>[4x]MLNSFKLSLQYILPKLWLTRLAGWGASKRAGWLTKLVIDLFVKYYKVDMKEAQKPDTASYRTFNEFFVRPLRDEVRPIDTDPNVLVMPADGVISQLGKIEEDKILQAKGHNYSLEALLAGNYLMADLFRNGTFVTTYLSPRDYHRVHMPCNGILREMIYVPGDLFSVNHLTAQNVPNLFARNERVICLFDTEFGPMAQILVGATIVGSIETVWAGTITPPREGIIKRWTWPAGENDGSVALLKGQEMGRFKLG;>XTVINLFAPGKVNLVEQLESLSVTKIGQPLAVSTGHHHHHHG[4x]

Phosphatidylethanolamine (PE), a major component of the cellular membrane across all domains of life, is synthesized exclusively by membrane-anchored phosphatidylserine decarboxylase (PSD) in most bacteria. PSD is translated as an inactive proenzyme and undergoes self-cleavage between a conserved Gly-Ser pair to become an active αβ-heterodimer. This maturation step results in the post-translational modification of the N-terminus serine to pyruvoyl in the α-subunit, which is an indispensable prosthetic group for decarboxylation activity. After the proenzyme undergoes auto-proteolysis, an active complex is formed between the α- and β-chains, which are mainly responsible for catalytic activity and membrane association, respectively.

To identify the molecular determinants required for substrate recognition and binding, we first attempted to form a stable covalent linkage between PSD and a phospholipid via sodium cyanoborohydride (NaCNBH3)-dependent reduction of a Schiff base intermediate. Among these samples, 8PE- and 10PE-linked PSD1–287 yielded crystals, which diffracted to 2.12 Å and 2.70 Å resolution, respectively. These X-ray diffraction data were used to determine the structures shown in Fig. 4C; they are further denoted as 8PE-PSD and 10PE-PSD, respectively. The overall conformation of PSD in both PE-bound structures is highly homologous to that in apo structures (r.m.s.d. of Cαs = 0.218 Å for 8PE-PSD; 0.399 Å and 0.390 Å for the 10PE-PSD αβ-heterotetramer). For instance, the entire sn-2 acyl chains could be modeled in 10PE-PSD, whereas most sn-1 acyl chains were disordered because of the relatively shallow binding pocket. In both structures, the sn-2 acyl chains extend to the hydrophobic surface of the N-terminal helical domain, where the membrane association is presumed to occur. The phosphate group of PE forms hydrogen bonds with the side chain of Tyr-137 and the backbone amide group of Val-167 in both PE-bound structures, and an additional hydrogen bond is identified with the side chain of Ser-166 in 10PE-PSD. The orientation of Pvl-254-linked PE in both structures suggests that His-144 is likely to interact with the departing carboxyl group of PS. Solid electron densities were observed in all subunits of PE connected to Pvl-254.> MSFTVDSARGIFPNTLTADVVPATIARFNQLNAEDQLALIWFAYLEMGKTITVAALGAANMQFAEITMNQIRQMSFQEQTQVMCDLANRTDTPISRAYGSWTANIKLGFWYQLGEWMAQGIVAPIPSGYKLS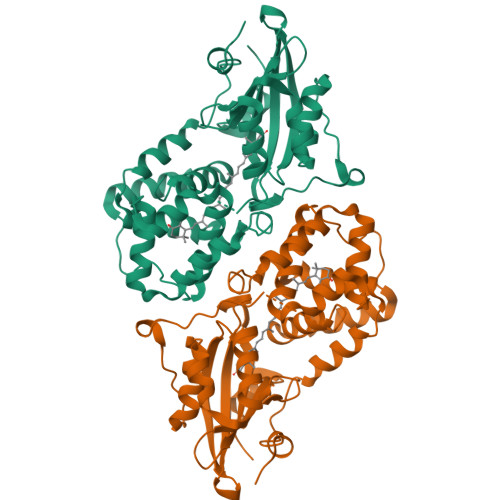ANAASVLQAIQGLESGQQITVLRNCVVDMGFDTSKLDSSQRVSEPVVVPRDMAQRTQVTIEGIDNPTVLNYMNNMNANDFEVLIELFTPDGALQPPFQKPIVGKDAVLRFFREECQNLKLIPERGVTEPADGGYTQIKVTGKVQTPWFGAGVGMNMAWRFLLSPENKIFFVAIDLLASPKELLNLVR> NEVKYPVVYEIFIRSLYDSDGDGVGDINGVSQKVDYLRKLGIDAVWFMPFNEAVSYHGYDITDYYNVEKDYGTMEDLENMIQVLHENGIKVIMDLVINHTSDEHPWFKDAVENTTSSPYWDYYIMSLEDHSGQDHWHWKINSKGQKVWYFGLFGYNMPDLNHDSQKVREEVKKIVDFWISKGVDGFRIDAAKHIYGWSWDDGIQESAEYFEWFRDYVLSKKPDAILVGEVFSGNTYDLSLYPIPVFNFALMYSIRNYPEGQDGMIENNWVEESFLFLENHDLHRFFSHLQEHYKKFSESDYEFIKKRAALWYFLIFTLKGSPVIYYGGEIGTRGFKWHGPVYDEPVREPMQWYASGTGEGQTFWTKEVYKNAGITFGNADVDGCIYDDPYDGFSVEEQENDPKSLLNFIRFILNFRKDHDAILNGDQTIFRDWKNLIAFYRESSNEKLLVVLNPDPVWQNSFTFEENMTMILEVDFENFIWNESNVSFSAGESFTVDPMKAYIFKK;> EVKYPVVYEIFIRSLYDSDGDGVGDINGVSQKVDYLRKLGIDAVWFMPFNEAVSYHGYDITDYYNVEKDYGTMEDLENMIQVLHENG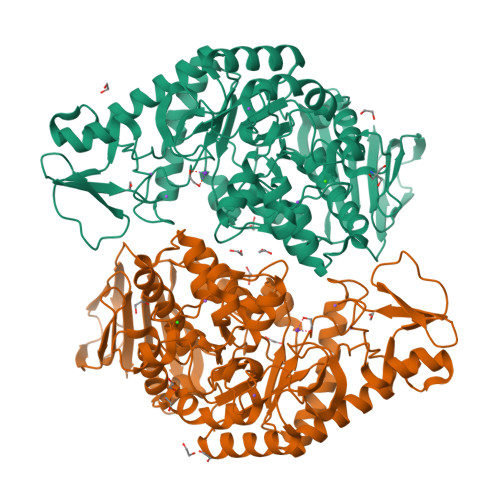IKVIMDLVINHTSDEHPWFKDAVENTTSSPYWDYYIMSLEDHSGQDHWHWKINSKGQKVWYFGLFGYNMPDLNHDSQKVREEVKKIVDFWISKGVDGFRIDAAKHIYGWSWDDGIQESAEYFEWFRDYVLSKKPDAILVGEVFSGNTYDLSLYPIPVFNFALMYSIRNYPEGQDGMIENNWVEESFLFLENHDLHRFFSHLQEHYKKFSESDYEFIKKRAALWYFLIFTLKGSPVIYYGGEIGTRGFKWHGPVYDEPVREPMQWYASGTGEGQTFWTKEVYKNAGITFGNADVDGCIYDDPYDGFSVEEQENDPKSLLNFIRFILNFRKDHDAILNGDQTIFRDWKNLIAFYRESSNEKLLVVLNPDPVWQNSFTFEENMTMILEVDFENFIWNESNVSFSAGESFTVDPMKAYIFKK>AGKTMIPLLAFAAWSGTGKTTLLKKLIPALCARGIRPGLIKHTHHDMDVDKPGKDSYELRKAGAAQTIVASQQRWALMTETPDEEELDLQFLASRMDTSKLDLILVEGFKHEEIAKIVLFRDGAGHRPEELVIDRHVIAVASDVPLNLDVALLDI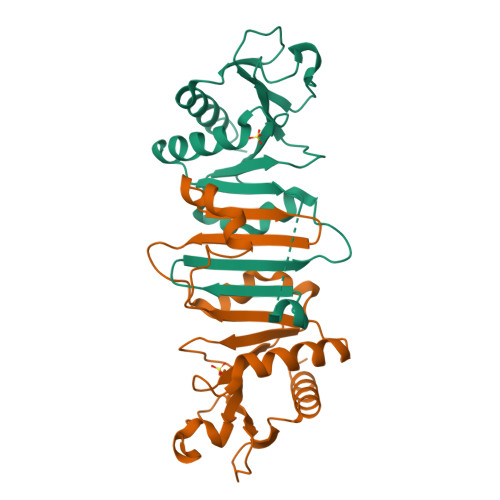NDVEGLADFVVEWMQKQNG[2x]>LNQSPLLINLDIDPVTGDSVINAAEAGGTVTLTGVVNGDVFSSGVVTLVINGVTYSTNVNPNGTWSVSVAGSDLSADSDRIVDASVVVTNGAGQQGTADSTESFIVKTSSRATIRVNSITSDDVVNAEESNSTITVSGRVGLDASAGDTVSMTINGTLYTTVVLANKTWSVGVSGSDLAQDNSFQVSVTGQDSAGNPYAGTTTSTHTVDTSADAGTVTVNAITSDDVINASEAAGTV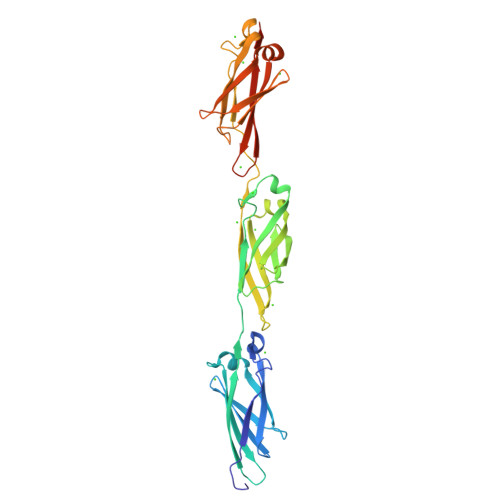AVSGTATGGDIAEGDTVTLEINGETYTTTVDANGEWSVDVAGSDLAADTAFDAVVTSSDAAGNTVDTTGSSTHTVDLEHHHHHH[2x]>[2x]MRTRSTISTPNGITWYYEQEGTGPDIVLVPDGLGECQMFDSSVSQIAAQGFRVTTFDMPGMSRSAKAPAETYTEVTAQKLASYVISILDALDIKHATVWGCSSGASTVVALLLGYPDRIRNAMCHELPTKLLDHLSNTAVLEDEEISNILANVMLNDVSGGSEAWQALGVEVHARLHKNYPVWARGYPRTIPPSAPVQDVEALRGKPLDWTVGAATPTESFFDNIVTATKAGVNIGLLPGMHFPYVSHPDVFAKYVVETTQKHLWNSSSVDKLAAALEHHHHHH

ZEN is a resorcylic acid lactone that is produced by several Fusarium species as an oestrogenic mycotoxin. Zearalenone hydrolase (ZHD) is an α/β-hydrolase that has been shown to be able to detoxify ZEN. Structures of apo ZHD and some enzyme–substrate complexes have recently been reported. These structures reveal a catalytic triad consisting of Ser102–His242–Glu126 inside a ZEN-binding tunnel that is enclosed by the α/β-hydrolase fold and a helical cap domain.

Here, we report the 1.60 Å resolution structure of a complex of ZHD with the hydrolytic product of zearalenone, which reveals the final stage of zearalenone hydrolysis. In order to obtain the enzyme–product complex structure, apo ZHD crystals were soaked in 2 mM ZEN for between 1 and 45 min before quenching in liquid nitrogen. The expected hydrolytic product ZGR did not appear until the crystals had been soaked for over 30 min. The crystals of our C-terminally His6-tagged ZHD protein diffracted to approximately 1.60 Å resolution, which is much better than the resolutions reported from structures crystallized using an N-terminally His6-tagged ZHD construct. The conjugated coplanar structure of ZGR was comprised of an entire phenol ring, an adjacent carbon double bond C1′=C2′ and a carboxyl group O12′=C12′—O13′. When the product (ZGR) complex was superimposed on the substrate (ZEN) complex, changes in the phenol-ring position were noted. Structural superposition of the ZHD/S102A–ZEN structure and our ZHD–ZGR structure revealed that Ser102 Oγ of the catalytic triad points towards the lactone C atom C12′ of the carboxyl group at a distance of 2.52 Å. This suggests that a nucleophilic attack on C12′ initiates the hydrolysis reaction. Taken together, we suggest that these interactions are altered as a result of the breakage of the lactone bond. It is very likely that Trp183 N∊1 is responsible for the unidirectional translational movement of the phenol ring, which in turn determines the conformational change of the lactone loop following cleavage of the lactone bond. In the case of ZHD, this enzyme–product structure provides the final state of catalysis.>MAQIAERLASLRSQLPPSVQLIAVSKNHPAAAIREAYAAGQRHFGENRVQEAIAKQAELTDLPDLTWHLLGKLQSNKARKAVEHFDWIHSVDSWALAERLDRIAGELGRSPKLCLQVKLLPDPNKAGWDPADLRAELPQL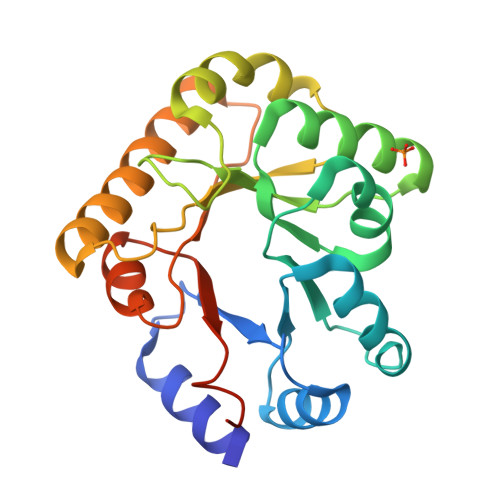SQLQQVQIRGLMVIAPLGLTAAETQALFAQARTFAAELQQQAPQLRLTELSMGMSSDWPLAVAEGATWIRVGTQLFGPRSLEHHHHHH[2x]>MTEDRLSAEDKKFLEVERALKEAALNPLRHATEELFGDFLKMENITEICYNGNKVVWVLKNNGEWQPFDVRDRKAFSLSRLMHFARCCASFKKKTIDNYENPILSSNLANGERVQIVLSPVTVNDETISISIRIPSKTTYPHSFFEEQGFYNLLDNKEQAISAIKDGIAIGKNVIVCGGTGSGKTTYIKSIMEFIPKEERIISIEDTEEIVFKHHKNYTQLFFGGNITSADCLKSCLRMRPDRIILGELRSSEAYDFYNVLCSGHKGTLTTLHAGSSEEAFIRLANMSSSNSAARNIKFESLIEGFKDLIDMIVHINHHKQCDEFYIKHR[6x];>GDKLHEIKQELKDL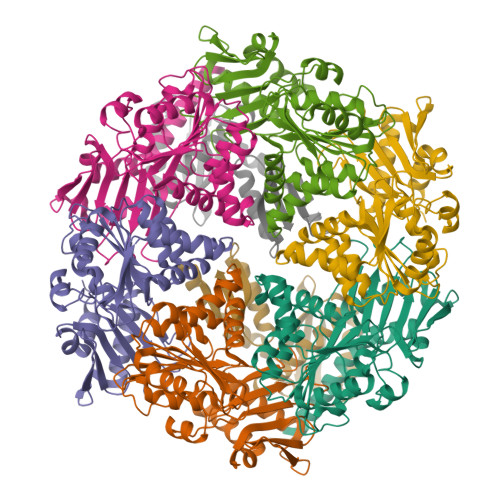FSHLPYKINKVEVSLYEPGVLLIDIDGEDSALLIGEKGYRYKALSYLLFNWIHPTYGYSIRLEISTFLQNQEKVMDTQLQSVIMTVHEVGKGQMKAPDGVLTYIALKKLRKAFPNKYVSIKTNLNDEKYIVINDFNNE[2x]The Notch receptor is a key component of a core metazoan signaling pathway activated by Delta/Serrate/Lag-2 ligands expressed on an adjacent cell. Notch signaling requires cell-surface expression of a hetero-dimeric transmembrane Notch receptor, which has a large extracellular portion rich in epidermal growth factor (EGF)-like domains (36 in human Notch1 and Drosophila Notch). Key to understanding receptor function is structural knowledge of the large extracellular portion of Notch which contains multiple repeats of epidermal growth factor (EGF)-like domains. Here we investigate the EGF4-13 region of human Notch1 (hN1) using a multidisciplinary approach.

We report a crystal structure of EGF4-7, where the domain interface formed between the non-Ca2+-binding domain, EGF6, and its preceding domain introduces a bent conformation to the region. Structures of two crystal forms (P21 and C2) were determined for hN1 EGF4-7 using X-ray crystallography. Each domain within the construct displayed a canonical EGF fold, with a single Ca2+ bound, as expected, to EGF5 and EGF7 (Handford et al., 1991, Mayhew et al., 1992, Rees et al., 1988). An unusual tilt angle of ∼80°–90° was observed at the domain interface of EGF5 and EGF6 for both crystal forms resulting in a bent conformation for this stretch of EGF domains. The EGF5-6 domain interface is stabilized in this orientation by packing of the side chain of A208 (with some contribution of T209) in EGF5 with V239 from EGF6. A second packing interaction is also evident between Y219 and P221 at the N terminus of EGF6. These interactions are very different from the interdomain packing typically observed in cbEGF-cbEGF pairs, and EGF-cbEGF pairs, which involves a conserved aromatic residue located between the fifth and sixth cysteine in the N-terminal domain packing against residues on the major β hairpin of the C-terminal domain, resulting in a rod-shaped conformation (Cordle et al., 2008a, Downing et al., 1996, Hambleton et al., 2004, Smallridge et al., 2003). H210, which is located at the position of the conserved packing aromatic residue in EGF5, is instead involved in an intradomain interaction with H191 that helps to stabilize the loop containing A208. The EGF4-5 and EGF6-7 pairs adopt a more elongated conformation than observed for EGF5-EGF6, but these pairs are not as elongated as the previously determined structure for EGF11-13. In solution, the EGF5-6 interface is also observed to be bent but is somewhat more open (70° ± 2°) than the crystal structures.

>QDPCASNPCANGGQCLPFEASYICHCPPSFHGPTCRQDVNECGEKPGLCRHGGTCHNEVGSYRCVCRATHTGPNCERPYVPCSPSPCQNGGTCRPTGDVTHECACLPGFTGQNCEENIDDCPGNNCKNGGACVDGVNTYNCRCPPEWTGQYCTE[2x]> GAMGKCPTKVVLLRNMVGAGEVDEDLEVETKEECEKYGKVGKCVIFEIPGAP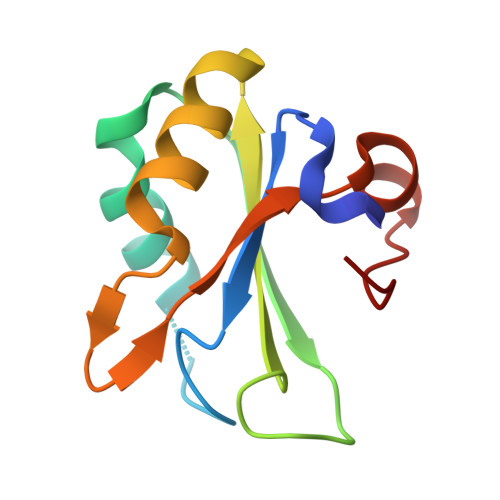DDEAVRIFLEFERVESAIKAVVDLNGRYFGGRVVKACFYNLDKFRVLDLAEQV>[2x]MAEKPKLHYFNARGL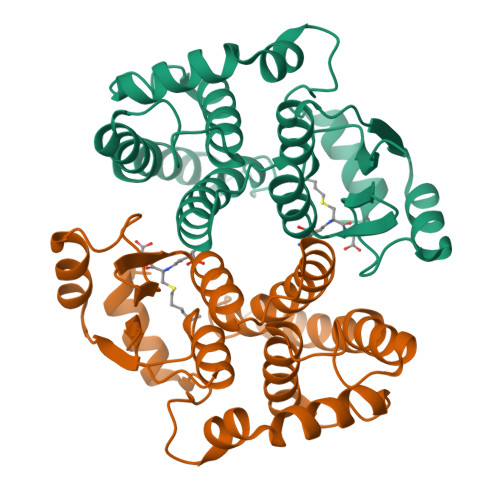MESTRWLLAAAGVEFEEKFIKSAEDLDKLRNDGYLMFQQVPMVEIDGMKLVQTRAILNYIASKYNLYGKDIKERALIDMYIEGIADLGEMILLLPVCPPEEKDAKLALIKEKIKNRYFPAFEKVLKSHGQDYLVGNKLSRADIHLVELLYYVEELDSSLISSFPLLKALKTRISNLPTVKKFLQPGSPRKPPMDEKSLEEARKIFRF5-(4-fluorophenyl)-2,3-dihydroxy-N-[2-[5-(2-methylpyridin-4-yl)-4H-1,2,4-triazol-3-yl]ethyl]benzamide 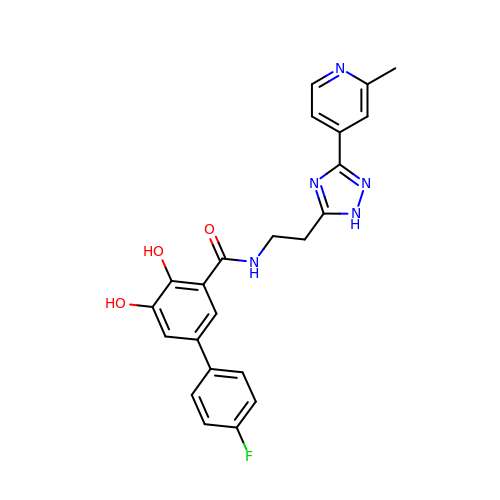| C23 H20 F N5 O3 | ZQNYOBSVRHHBCA-UHFFFAOYSA-N>SMNKPTMSFKDYI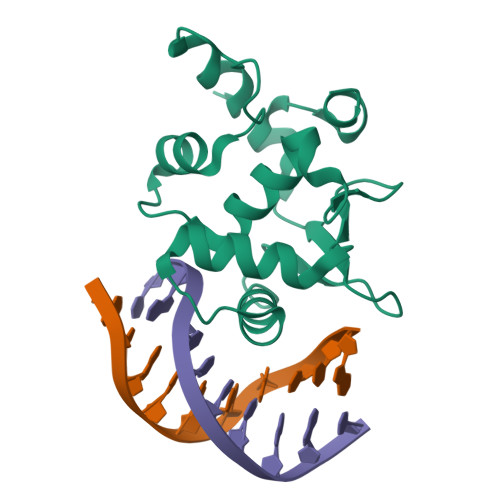QERSDPVEQGKPVIPAAVLAGFTGSGPIQLWQFLLELLSDKSCQSFISWTGDGWEFKLADPDEVARRWGKRKNKPKMNYEKLSRGLRYYYDKNIIHKTSGKRYVYRFVCDLQNLLGFTPEELHAILGVQ[3x]>MSNIQNMSLEDIMGERFGRYSKYIIQDRALPDIRDGLKPVQRRILYSMNKDSNTFDKSYRKSAKSVGNIMGNFHPHGDSSIYDAMVRMSQNWKNREILVEMHGNNGSMDGDPPAAMRYTEARLSEIAGYLLQDIEKKTVPFAWNFDDTEKEPTVLPAAFPNLLVNGSTGISAGYATDIPPHNLAEVIDAAVYMIDHPTAKIDKLMEFLPGPDFPTGAIIQGRDEIKKAYETGKGRVVVRSKTEIEKLKGGKEQIVITEIPYEINKANLVKKIDDVRVNNKVAGIAEVRDESDRDGLRIAIELKKDANTELVLNYLFKYTDLQINYNFNMVAIDNFTPRQVGIVPILSSYIAHRREVILARSRFDKEKAEKRLHIVEGLIRVISILDEVIALIRASENKADAKENLKVSYDFTEEQAEAIVTLQLYRLTNTDVVVLQEEEAELREKIAMLAAIIGDERTMYNLMKKELREVKKKFATPRLSSLEDTAKALEHHHHHH[2x];>MGHHHHHHHHHHSSGHIDDDDKHMKNKKDKGLLSGKLTPAQSKNPAKNELYLVEGDSAGGSAKQGRDRKFQAILPLRGKVINTAKAKMADILKNEEINTMIYTIGAGVGADFSIEDANYDKIIIMTDADTDGAHIQTLLLTFFYRYMRPLVEAGHV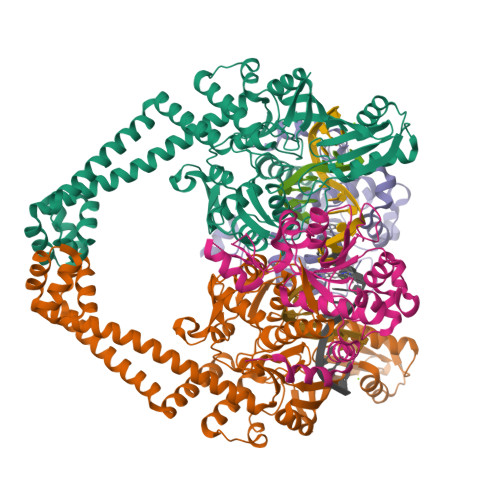YIALPPLYKMSKGKGKKEEVAYAWTDGELEELRKQFGKGATLQRYKGLGEMNADQLWETTMNPETRTLIRVTIEDLARAERRVNVLMGDKVEPRRKWIEDNVKFTLEEATVF[2x]2-{[(6-OXO-1,6-DIHYDROPYRIDIN-3-YL)METHYL]AMINO}-N-[4-PROPYL-3-(TRIFLUOROMETHYL)PHENYL]BENZAMIDE 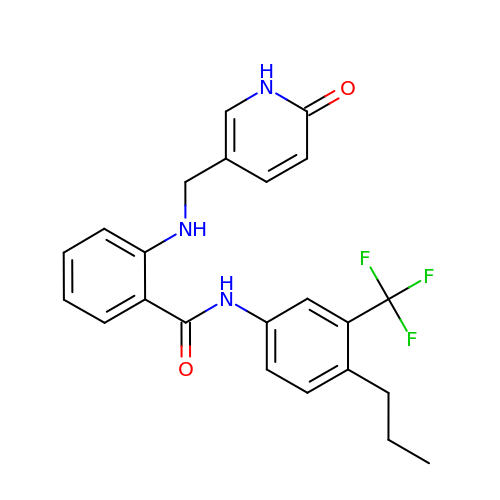| C23 H22 F3 N3 O2 | SHSORWZDEKFFLP-UHFFFAOYSA-N> GRLAGLSAALLRTDSFVGGRWLPAAATFPVQDPASGAALGMVADCGVREARAAVRAAYEAFCRWREVSAKERSSLLRKWYNLMIQNKDDLARIITAESGKPLKEAH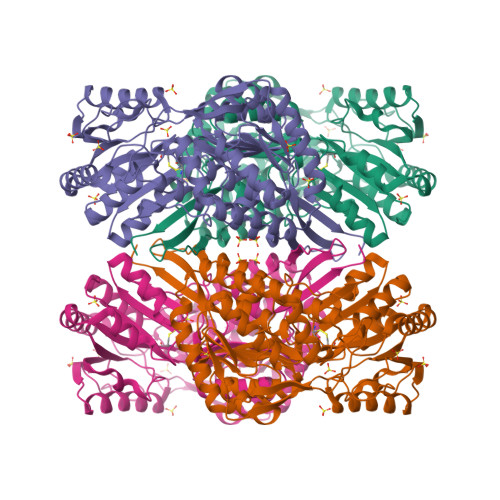GEILYSAFFLEWFSEEARRVYGDIIHTPAKDRRALVLKQPIGVAAVITPWNFPSAMITRKVGAALAAGCTVVVKPAEDTPFSALALAELASQAGIPSGVYNVIPCSRKNAKEVGEAICTDPLVSKISFTGSTTTGKILLHHAANSVKRVSMELGGLAPFIVFDSANVDQAVAGAMASKFRNTGQTCVCSNQFLVQRGIHDAFVKAFAEAMKKNLRVGNGFEEGTTQGPLINEKAVEKVEKQVNDAVSKGATVVTGGKRHQLGKNFFEPTLLCNVTQDMLCTHEETFGPLAPVIKFDTEEEAIAIANAADVGLAGYFYSQDPAQIWRVAEQLEVGMVGVNEGLISSVECPFGGVKQSGLGREGSKYGIDEYLELKYVCYGGL>MKGDQKVIEYLNRGLRSELTAVSQYWLHYRMLEDWGYKDLAKKWRAESIEEMAHADKFVERILFLEGLPNLQTLDPLRIGQTVKEVLESDLAAEREARALYQEGAAYAASVGDFPSKNLFEELMGDEEHHIDFLETQLDLVSKLGLELYAQHHIGKLDD[2x]

Bacterioferritins (Bfr) solve two important problems for bacterial cells: they reduce the concentration of toxic free Fe(II), a source of reactive oxygen species through the Fenton reaction, and provide an accessible storage of iron in a mineralized ferric form. Bacterioferritins also possess 12 heme-b molecules intercalated between the protein subunits, this is the main feature that distinguishes them from eukaryotic ferritins. Here we report the crystal structure of bacterioferritin from Blastochloris viridis (Bv Bfr) up to 1.58 Å resolution. In Bv Bfr the ferroxidase active site consists of highly conserved amino acids: His54 and Glu18 are terminal ligands to iron 1 (Fe1), His130 and Glu94 are terminal ligands to iron 2 (Fe2), and Glu127 and Glu51 are bridging ligands.

Bacterioferritin from Blastochloris viridis was isolated from its native host and crystallized. Native crystals Bv Bfr diffracted to 1.8 Å resolution. In the “as-isolated” structure the ferroxidase center is fully occupied at the Fe1 site and 40% occupied at Fe2. Non-ligated conformation of His130 was not observed in any of the “as isolated” and “Fe(II)-soaked” crystal structures. The iron-iron distance is 3.97 Å for the native, “as isolated” protein, 3.81 Å in the Fe-soaked and 3.92 Å in the double soaked structure. A long iron-iron distance such as that observed in native and double soaked Bv Bfr, has been reported when the irons are reduced and not bridged by any electron density. In the “as isolated” and “double soaked” Bv Bfr the ligand-Fe1 distance is located within this range, while the ligand-Fe2 distance is longer, making the ligand interaction with Fe1 and Fe2 slightly weaker and more symmetric. We expected our aerobically isolated crystals to be in a fully oxidized state with an empty ferroxidase active site, but absorption spectra showed that the hemes-b are in a predominantly reduced state as judged from the sharp peak at 558 nm, although a shoulder at 564 nm indicates that a fraction of hemes are oxidized (black curve). The spectroscopic signature after X-ray data collection is unchanged (red curve), hence our structure of ‘as isolated’ Bfr contains mostly hemes in the reduced state. The ferroxidase active site is blocked for irons in the native state, but becomes instable upon “double soaking” treatment.> AGPEEHKARVEEYMRRALQAT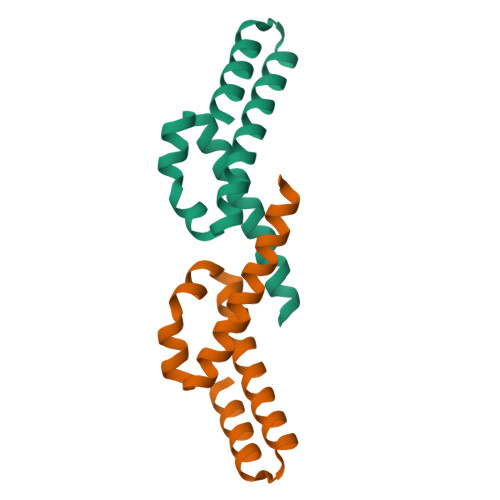TEPEKKYWEEEAKKEIEQAMYADALINPIRFTEKAAKYIKTYGFRGQEAYDQVKKEMFEKLYKYFMEKLKSE> GARSSSYSGEYGSGGGKRFSHSGNQLDGPITALRVRVNTYYIVGLQ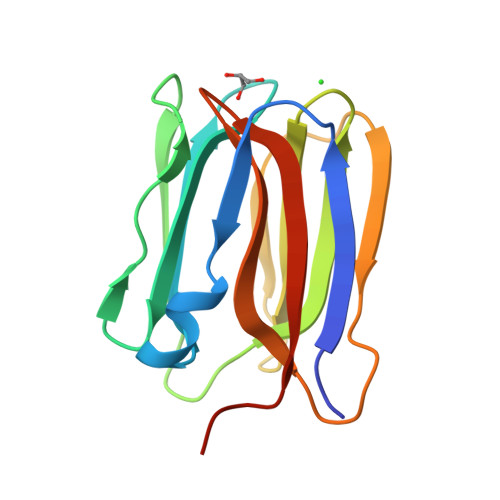VRYGKVWSDYVGGRNGDLEEIFLHPGESVIQVSGKYKWYLKKLVFVTDKGRYLSFGKDSGTSFNAVPLHPNTVLRFISGRSGSLIDAIGLHWDVYPTSCSRC>[4x]SNALTRQAQ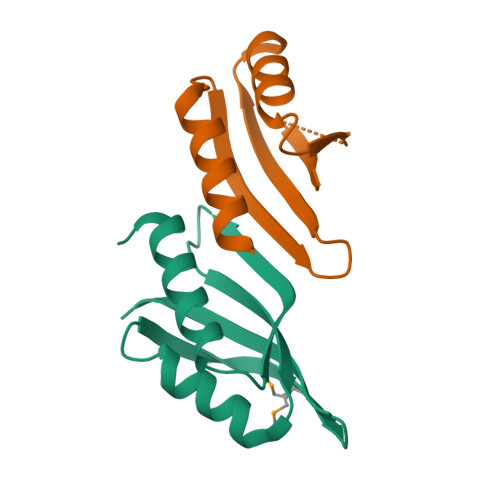HAPLVDRLSALQNILSETPGIRLRALSWDAAGNRLQLDIAAVSSRALEQFTQRAQPRFRVRPGDMITKPDGIEGQLTLEENDG> EQQRFPQRYIELAIVVDHGMYTKYSSNFKKIRKRVHQMVSNINEMCRPLNIAITLALLDVWSEKDFITVQADAPTTAGLFGDWRERVLLKKKNHDHAQLLTDTNFARNTIGWAYVGRMCDEKYSVAVVKDHSSKVFMVAVTMTHELGHNLGMEHDDKDKCKCDTCIMSAVISDKQSKLFSDCS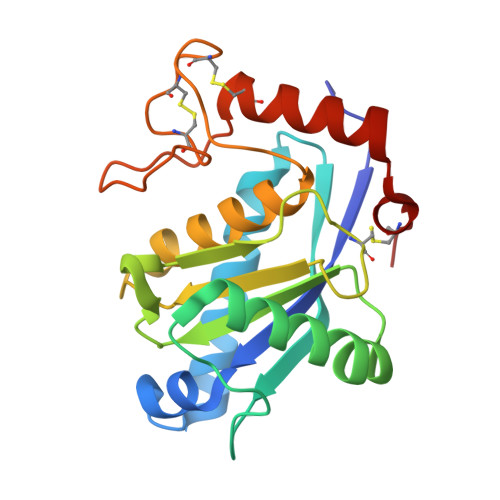KDYYQTFLTNDNPQCILNAP> MAFTRRQVLGGLVGLGVVGLGAGGVRYWLGRPESAVTHDYELIAAPVDMELVPGHVTPAWGYGGQAPGVELRCRQGDWLRVRFINKLDEPTTIHWHGIRLPLEMDGVPYVSQLPVQPGEYFDYVFKTEDAGNFWYHPHESSASQLGRGLVGPLVVEEREPSGFRHELSLSLKTWHVDEQGAFTPFMVPREAAREGTRGRLTTVNARPNPTLELPAGQVVRLRLFNLDNTVTYRLNLPGAEARLYALDGHPIEPRPLGKEYWLGPGMRIDLAVRVPE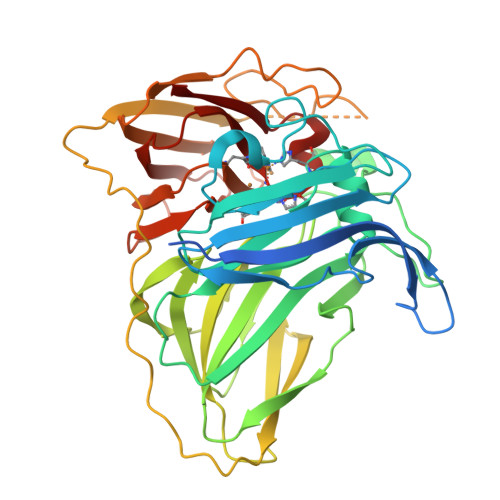AGRELPLRNGPLRLATLKSVASVEAPGDWPAPLPANPVAEPDLSIAETLSFRFEWAATLVDNLAQGGSYKYWQINGQAWDINDISCAERPIATLKKGGHYIFELRNLAQYQHPIHLHGMVFKVLSSDRREIIPYFTDTYLLGKNETARVALVADNPGVWMFHCHVIDHMETGLMAAIEVA2,3-bis(bromomethyl)quinoxaline 1,4-dioxide | C10 H8 Br2 N2 O2 | 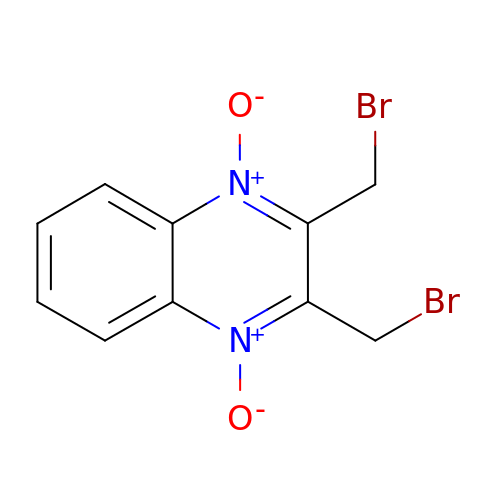DQKNFTLRMZOAMG-UHFFFAOYSA-N>[6x]GSPLPAAGFKKQQRKFQYGNYCKYYGYRNPSCEDGRLRVLKPEWFRGRDVLDLGCNVGHLTLSIACKWGPSRMVGLDIDSRLIHSARQNIRHYLSEELRLP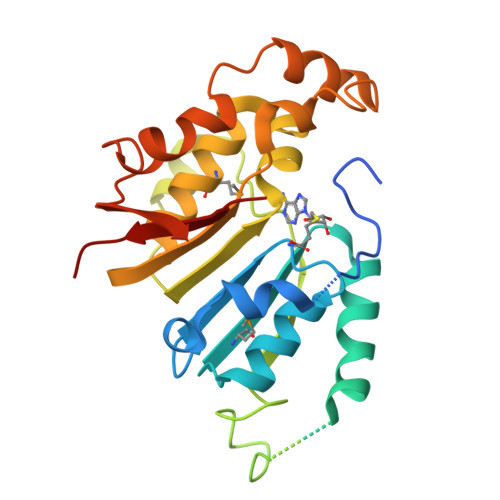PQTLEGDPGAEGEEGTTTVRKRSCFPASLTASRGPIAAPQVPLDGADTSVFPNNVVFVTGNYVLDRDDLVEAQTPEYDVVLCLSLTKWVHLNWGDEGLKRMFRRIYRHLRPGGILVLEPQPWSSYGKRKTLTETIYKNYYRIQLKPEQFSSYLTSPDVGFSSYELVATPHNTSKGFQRPVYLFHKARSPSH> 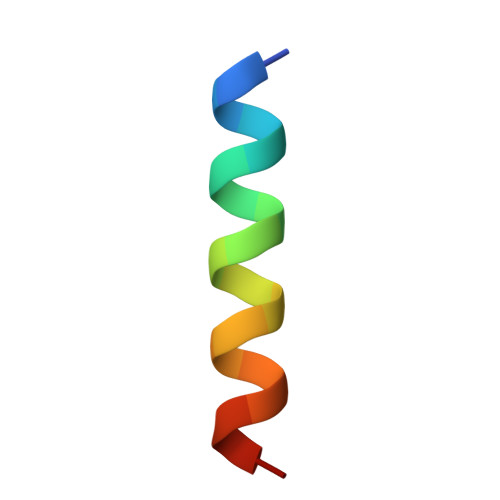DEHELLETAARWFYEIAKRA~{N}-[4-(3-chlorophenyl)-5-(2-chlorophenyl)carbonyl-1,3-thiazol-2-yl]-2-(4-ethylsulfonylphenyl)ethanamide 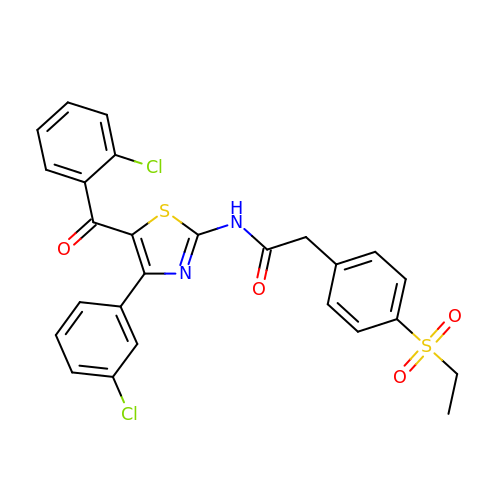| C26 H20 Cl2 N2 O4 S2 | GRWNPFJXINLSNF-UHFFFAOYSA-N>MASQPNSSAKKKEEKGKNIQVVVRCRPFNLAERKASAHSIVECDPVRKEVSVRTGGLADKSSRKTYTFDMVFGASTKQIDVYRSVVCPILDEVIMGYNCTIFAYGQTGTGKTFTMEGERSPNEEYTWEEDPLAGIIPRTLHQIFEKLTDNGTEFSVKVSLLEIYNEELFDLLNPSSDVSERLQMFDDPRNKRGVIIKGLEEITVHNKDEVYQILEKGAAKRTTAATLMNAYSSRSHSVFSVTIHMKETTIDGEELVKIGKLNLVDLAGSENIGRSGAVDKRAREAGNINQSLLTLG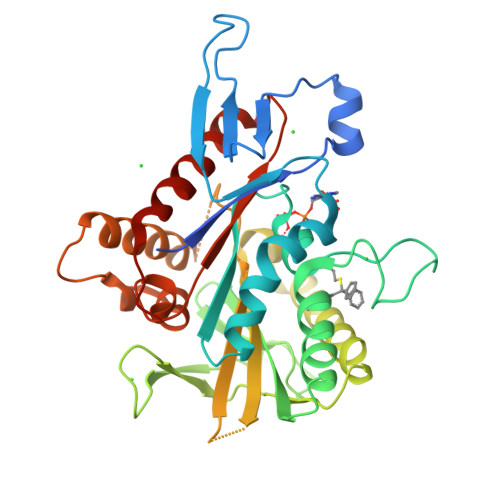RVITALVERTPHVPYRESKLTRILQDSLGGRTRTSIIATISPASLNLEETLSTLEYAHRAKNILNKPEVNQK[7x]> GIDPFTSDKIDEMYDIFGDGHDYDWALEIENEELENGNDNNEAE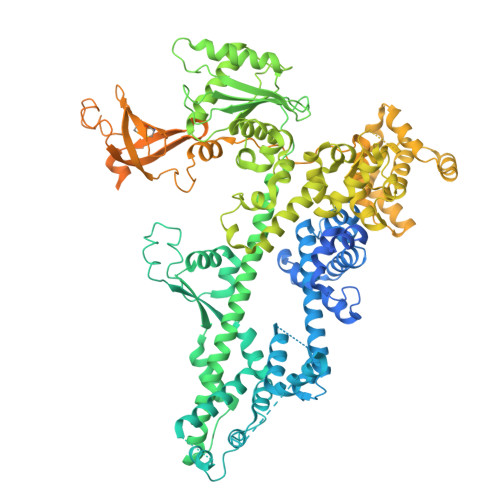EEEIDEETGAIKSTKKKISLQDIYDLEDLKKNLMTEGDMKIRKTDIPERYQELRAGITDYGNMSSEDQELERNWIAEKISVDKNFDANYDLTEFKEAIGNAIKFITKENLEVPFIYAYRRNYISSREKDGFLLTEDDLWDIVSLDIEFHSLVNKKDYVQRFYAELHIDDPIVTEYFKNQNTASIAELNSLQDIYDYLEFKYANEINEMFINHTGKTGKKHLKNSSYEKFKASPLYQAVSDIGISAEDVGENISSQHQIHPPVDHPSSKPVEVIESILNANSGDLQVFTSNTKLAIDTVQKYYSLELSKNTKIREKVRSDFSKYYLADVVLTAKGKKEIQKGSLYEDIKYAINRTPMHFRRDPDVFLKMVEAESLNLLSVKLHMSSQAQYIEHLFQIALETTNTSDIAIEWNNFRKLAFNQAMDKIFQDISQEVKDNLTKNCQKLVAKTVRHKFMTKLDQAPFIPNVRDPKIPKILSLTCGQGRFGADAIIAVYVNRKGDFIRDYKIVDNPFDKTNPEKFEDTLDNIIQSCQPNAIGINGPNPKTQKFYKRLQEVLHKKQIVDSRGHTIPIIYVEDEVAIRYQNSERAAQEFPNKPPLVKYCIALARYMHSPLLEYANLTSEEVRSLSIHPHQNLLSSEQLSWALETAFVDIVNLVSVEVNKATDNNYYASALKYISGFGKRKAIDFLQSLQRLNEPLLARQQLITHNILHKTIFMNSAGFLYISWNEKRQKYEDLEHDQLDSTRIHPEDYHLATKVAADALEYDPDTIAEKEEQGTMSEFIELLREDPDRRAKLESLNLESYAEELEKNTGLRKLNNLNTIVLELLDGFEELRNDFHPLQGDEIFQSLTGESEKTFFKGSIIPVRVERFWHNDIICTTNSEVECVVNAQRHAGAQLRRPANEIYEIGKTYPAKVIYIDYANITAEVSLLDHDVKQQYVPISYSKDPSIWDLKQELEDAEEERKLMMAEARAKRTHRVINHPYYFPFNGRQAEDYLRSKERGEFVIRQSSRGDDHLVITWKLDKDLFQHIDIQELEKENPLALGKVLIVDNQKYNDLDQIIVEYLQNKVRLLNEMTSSEKFKSGTKKDVVKFIEDYSRVNPNKSVYYFSLNHDNPGWFYLMFKINANSKLYTWNVKLTNTGYFLVNYNYPSVIQLCNGFKTLLKSNSSKNRMNNYR7-[[3-[2-(dimethylamino)ethyl]phenoxy]methyl]quinolin-2-amine | C20 H23 N3 O | 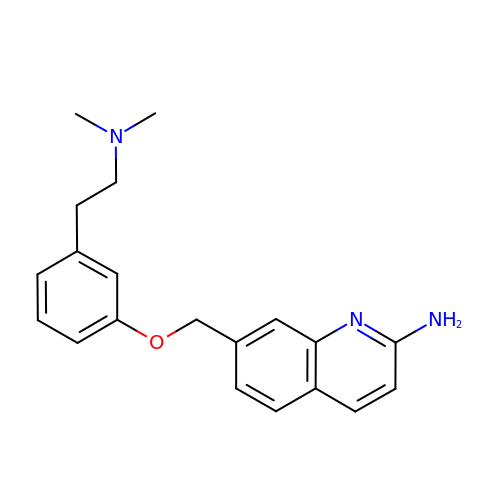TTZAIJYOUAIUID-UHFFFAOYSA-N>MII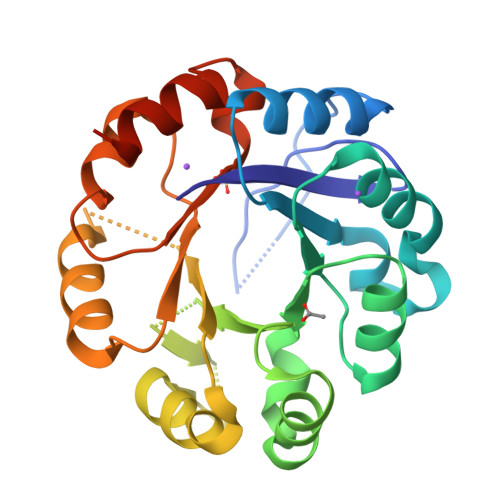PALDLIGGTVVRVVRLHQGDYARLRDYGNDPLPRLQDYAAQGAGVLHLVDLTGAKDPAKRQIPLIKTLVAGVNVPVQVGGGVRTEEDVAALLKAGVARVVIASTALKSPDVVKGWFERFGAQALVLALDVRIDEHGTKQVAVSGWQENSGVSLEQLVETYLPVGLKHVLCTDISRDGTLAGSNVSLYEEVCARYPQIAFQSSGGIGDIDDIAALRGTGVRGVIVGRALLEGKFTVKEAIQCWQNVKGHHHHHH[2x]>[3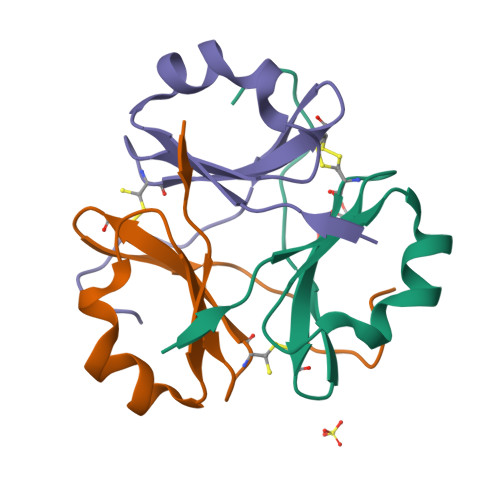x]GGSSGVRLWATRQAMLGQVHEVPEGWLIFVAEQCELYVRCQNGFRKVQLEARTPLPR>MSVDYPRDLIGYGSNPPHPHWPGKARIALSFVLNYEEGGERNILHGDKESEAFLSEMVSAQPLQGERNMSMESLYEYGSRAGVWRILKLFKAFDIPLTIFAVAMAAQRHPDVIRAMVAAGHEICSHGYRWIDYQYMDEAQEREHMLEAIRILTELTGERPLGWYTGRTGPNTRRLVMEEGGFLYDCDTYDDDLPYWEPNNPTGKPHLVIPYTLDTNDMRFTQVQGFNKGDDFFEYLKDAFDVLYAEGAEAPKMLSIGLHCRLIGRPARLAALQRFIEYAKSHEQVWFTRRVDIARHWHATHPYTG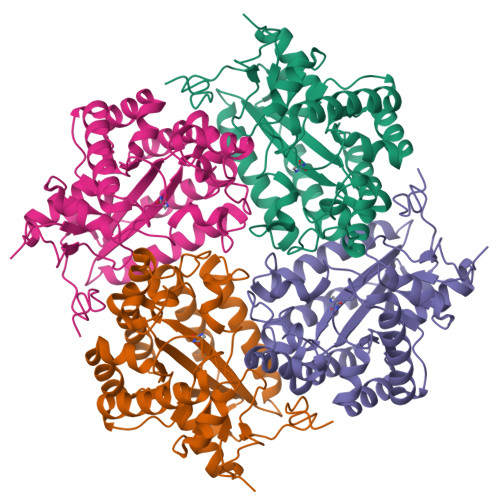AAK[2x]>[2x]MAIGEFMVSLPRMVYPQPKVLTPCRKDVLVVTPWLAPIVWEGTFNIDILNEQFR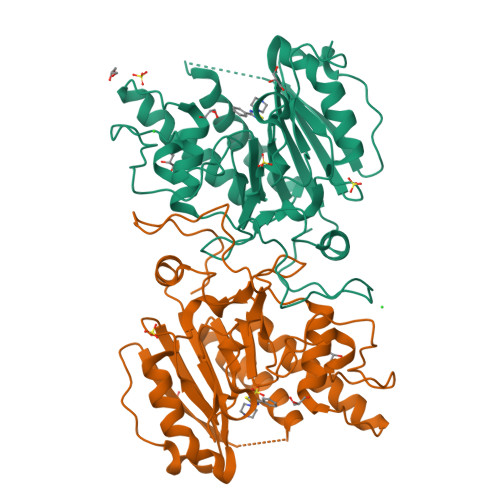LQNTTIGLTVFAIKKYVAFLKLFLETAEKHFMVGHRVHYYVFTDQPAAVPRVTLGTGRQLSVLEVRAYKRWQDVSMRRMEMISDFCERRFLSEVDYLVCVDVDMEFRDHVGVEILTPLFGTLHPSFYGSSREAFTYERRPQSQAYIPKDEGDFYYMGAFFGGSVQEVQRLTRACHQAMMVDQANGIEAVWHDESHLNKYLLRHKPTKVLSPEYLWDQQLLGWPAVLRKLRFTAVPKNHQAVRNP> MWSSLFGWTSSNAKNKESPTKAIVRLREHINLLSKKQSHLRTQITNQENEARIFLTKGNKVMAKNALKKKKTIEQLLSKVEGTMESMEQQLFSIESANLNLETMRAMQEGAKAMKTIHSGLDIDKVDETMDEIREQVELGDEISDAISRPLITGANEVDEDELDEELDMLAQENANQETSKIVNNNVNAAPISENKVSLPSVPSNKIKQSENSV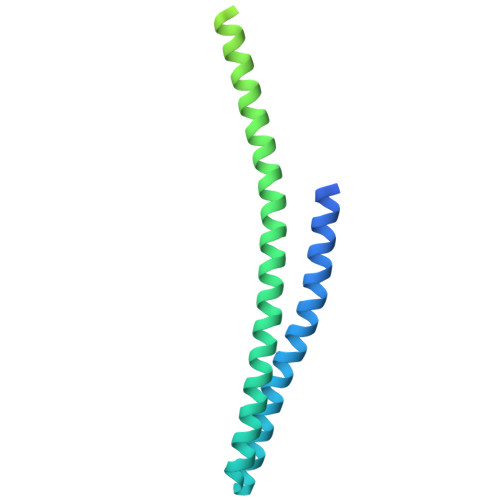KDGEEEEDEEDEDEKALRELQAEMGL1-METHYL-4-[4-[4-(4-(1-METHYLQUINOLINIUM)AMINO)BENZAMIDO]ANILINO]PYRIDINIUM 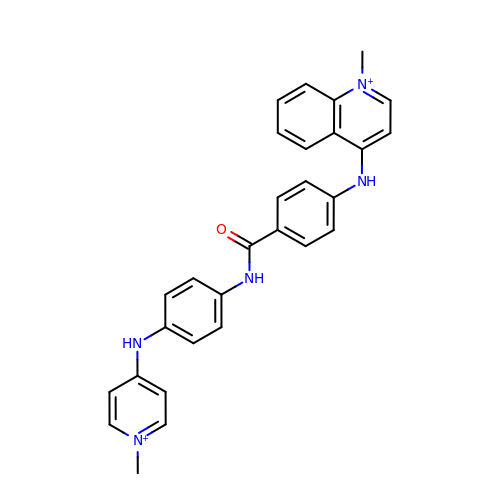| C29 H27 N5 O | PMCURUPNDHFYCG-UHFFFAOYSA-P> CYHGNGQSYRGTFSTTVTGRTCQSWSSMTPHRHQRTPENYPNDGLTMNYCRNPDADTGPWCFTMDPSIRWEYC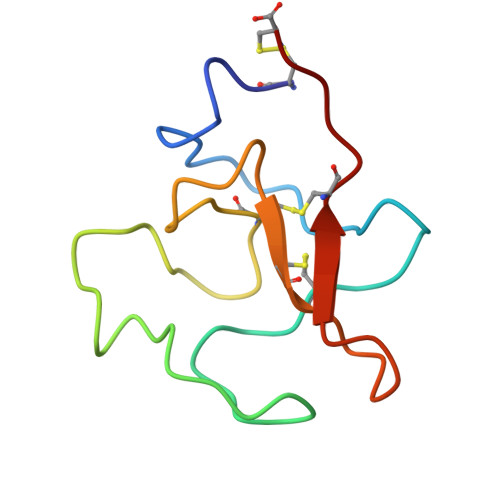NLTRC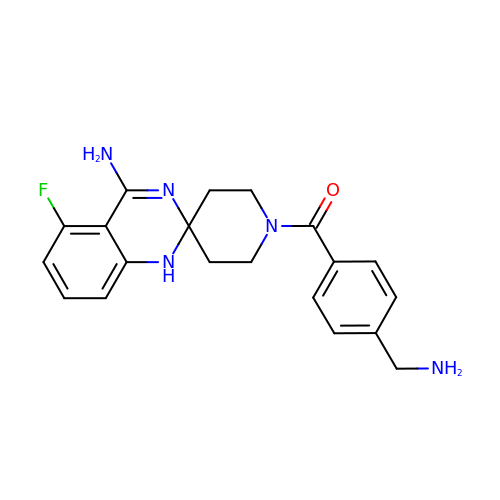1-[4-(AMINOMETHYL)BENZOYL]-5'-FLUORO-1'H-SPIRO[PIPERIDINE-4,2'-QUINAZOLIN]-4'-AMINE | C20 H22 F N5 O | SFPCNWQWKOUNRT-UHFFFAOYSA-N>[2x]GAMEGIKVFLH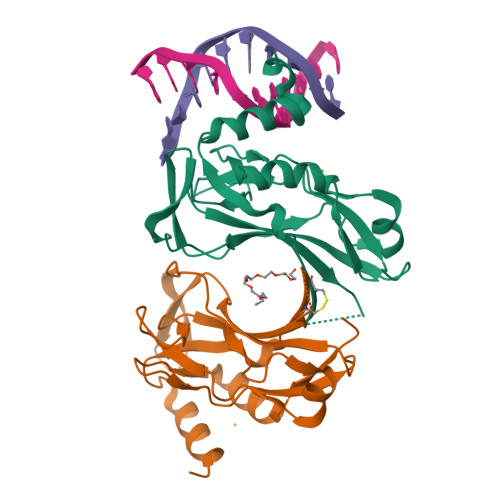ERELWLKFHEVGTEMIITKAGRRMFPSYKVKVTGLNPKTKYILLMDIVPADDHRYKFADNKWSVTGKAEPAMPGRLYVHPDSPATGAHWMRQLVSFQKLKLTNNHLDPFGHIILNSMHKYQPRLHIVKADENNGFGSKNTAFCTHVFPETAFIAVTSYQNHKITQLKIENNPFAKGFRGSDDMELHRMSRMQ>[4x]VANPEHYIKHPLQNRWALWFFKNDKSKTWQANLRLISKFDTVEDFWALYNHIQLSSNLMPGCDYSLFKDGIEPMWEDEKNKRGGRWLITLNKQQRRSDLDRFWLETLL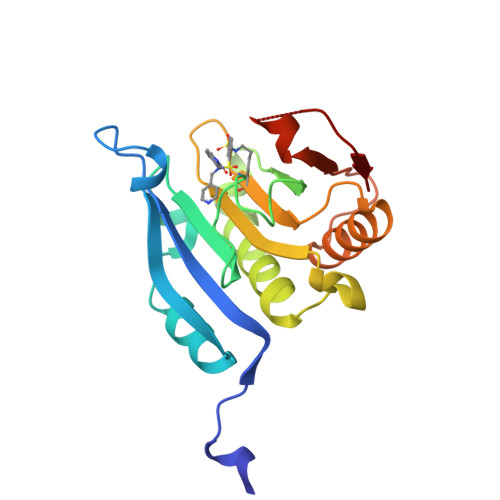CLIGESFDDYSDDVCGAVVNVRAKGDKIAIWTTECENRDAVTHIGRVYKERLGLPPKIVIGYQSHADTATKSGSTTKNRFVV>EMCEIPEMDSHLVEKLGQHLLPWMDRLSLEHLNPSIYVGLRLSSLQAGTKEDLYLHSLKLGYQQCLLGSAFSEDDGDCQGKPSMGQLALYLLALRANCEFVRGHKGDRLVSQLKWFLEDEKRAIGHDHKGHPHTSYYQYGLGILALCLHQKRVHDSVVDKL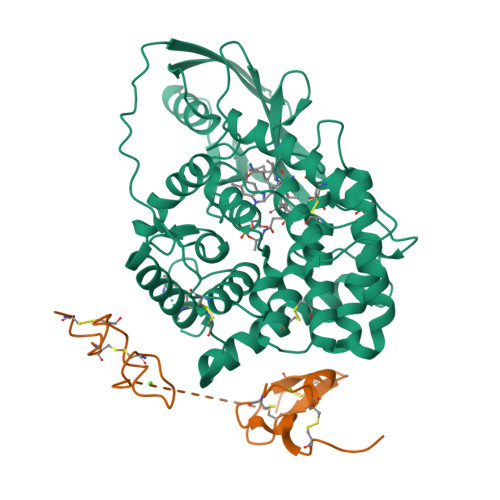LYAVEPFHQGHHSVDTAAMAGLAFTCLKRSNFNPGRRQRITMAIRTVQEEILKAQTPEGHFGNVYSTPLALQFLMTSPMRGAELGTACLKARVALLASLQDGAFQNALMISQLLPVLNHKTYIDLIFPDCLAPRVMLEPAAETIPQTQEIISVTLQVLSLLPPYRQSISVLAGSTVEDVLKKAHELGGFTYETQASLSGPYLTSVMGKAAGEREFWQLLRDPNTPLLQGIADYRPKDGETIELRLVSW[2x];>[2x]SCPPTKFQCRTSGLCVPLTWRCDRDLDCSDGSDEECRIEPCTQKGQCPPPPGLPCPCTGVSDCSGGTDKKLRNCSRLACLAGELRCTLSDDCIPLTWRCDGHPDCPDSSDELGCGTNE1-(PHENYLMETHYL)CYCLOPENTYL[(1S)-1-FORMYLPENTYL]CARBAMATE 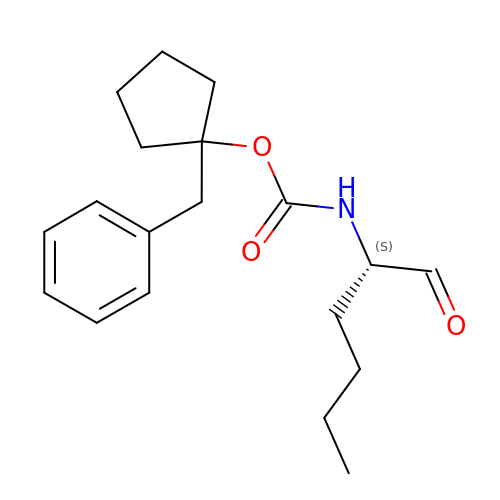| C19 H27 N O3 | ONABDOMWRCXLPX-KRWDZBQOSA-N> MPTLFDPIDFGPIHAKNRIVMSPLTRGRADKEAVPTPIMAEYYAQRASAGLIITEATGISREGLGWPFAPGIWSDAQVEAWKPIVAGVHAKGGKIVCQLWHMGRMVHSSVTGTQPVSSSATTAPGEVHTYEGKKPFEQARAIDAADISRILNDYENAARNAIRAGFDGVQIHAANGYLIDEFLRNGTNHRTDEYGGVPENRIRFLKEVTERVIAAIGADRTGVRLSPNGDTQGCIDSAPETVFVPAAKLLQDL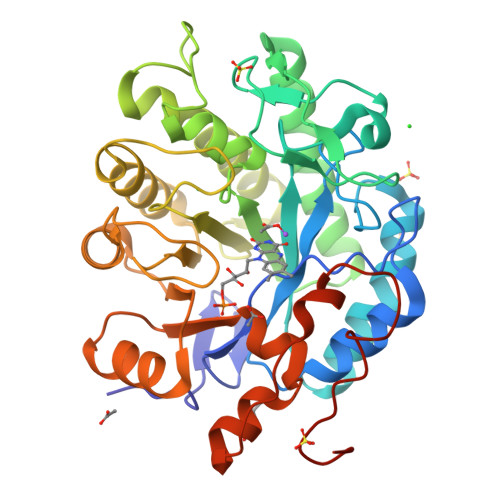GVAWLELREPGPNGTFGKTDQPKLSPQIRKVFLRPLVLNQDYTFEAAQTALAEGKADAIAFGRKFISNPDLPERFARGIALQPDDMKTWYSQGPEGYTDYPSATSGPNLEHHHHHH>QLQQQEDDRILGLPGQPNGVAFGMYGGYVTIDDNNGRALYYWFQEADTADPAAAPLVLWLNGGPGCSSIGLGAMQELGAFRVHTNGESLLLNEYAWNKAANILFAESPAGVGFSYSNTSSDLSMGDDKMAQDTYTFLVKWFERFPHYNYREFYIAGESGHFIPQLSQVVYRNRNNSPFINFQGLLVSSGLTNDHEDMIGMFESWWHHGLISDETRDSGLKVCPGTSFMHPTPECTEVWNKALAEQGNINPYTIYTPTCDREPSPYQRRFW[2x];>LPPYDPCAVFNSINYLNLPEVQTALHANVSGIVEYPWTVCSNTIF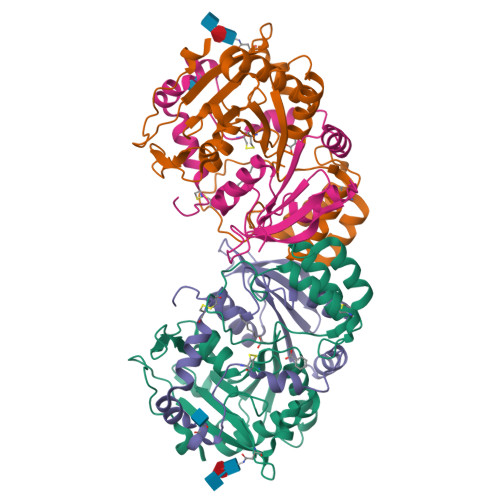DQWGQAADDLLPVYRELIQAGLRVWVYSGDTDSVVPVSSTRRSLAALELPVKTSWYPWYMAPTEREVGGWSVQYEGLTYVTVRGAGHLVPVHRPAQAFLLFKQFLKGEPMPAE[2x]> SMIEDVSLPSQVLQDQRLKELNQQLQDQLAQQTPYQNTKPLQDFKHLVVEESPCVTVKEISLIPLIGQSESDLQQFNFVIKAIKKHPQNILGKCIGTQSLHNIVNYAQNELLKKGFITSQIVVSPQDLNHGNLNLSIQIGRLNKIVIQEGKISSLQLKTGLPFKAGDIVNLKRLDQGLENLKRVYAVDMQITPATAQDKELTGYSDLILKLQALQKVNFNLSVDDSGNQDTGTYMGNIGIGINNPFHLNDILSLNVSHSLDDFHESLNRSYFISYQLPVGYYDLGFSYNDYQYRQGTVAPESGYPVIYHGNSQQANLNLSRVISRSGQHKTSVYGKLYHKESQSFLNDIEINVLHRKTSGWNLGVQHRQYLGNAVLDGSIDYRRGMGVGARTAPEENITDVYGNHLPVEGYSRAPLWSADLRYTTPFLLLDKPAQYRLNWRGQYAPKILVPNDRFYIGGRYSVRGFDGELMLSGDNGQYVQQEISLNAPIPNTQFYMAVDQGWVNGRNSIPGQRYLLGSVLGLRTYQNSFYLDAFTGRGLIAPDSIKKDWVTGFSINLSY

CdiB is an outer membrane transporter that releases its CdiA toxin to the cell surface. CdiB proteins are members of the Omp85 superfamily. Despite low sequence similarity (21% sequence identity), both structures adopt a common fold: an N-terminal α-helix (H1) is inserted into the lumen of the β-barrel and is connected by a ~ 20 residue linker to two periplasmic POTRA domains.

We determined two full-length crystal structures of CdiB transporters from Acinetobacter baumannii (strain ACICU) and E. coli (strain EC93), which will be referred to as CdiBAb and CdiBEc. CdiBAb and CdiBEc structures were built and refined to final resolutions of 2.4 Å and 2.6 Å, respectively. However, H1 is positioned very differently in CdiBAb and CdiBEc: the angle between H1 and the β-barrel is about 10° for CdiBAb, versus 25° for CdiBEc. In addition, H1 sits higher in the barrel pore in CdiBAb, positioning its N-terminus closer to the extracellular surface. In this orientation, H1 interacts with the inner barrel wall using 12 H-bonds and three salt bridges, with no interactions to loop 6, for a total buried surface area of 1263 Å2 (Figure 2—source data 1). In CdiBAb, the DxxG motif accounts for four residues on the 12-residue β1 strand, allowing β1 to form an extended β-sheet with β2, β3, and β16. As a result, the β-barrel is in a fully zipped conformation, stabilized by 10 H-bonds between strands β1 and β16. Extracellular loops 1–2 are short, with loop 2 curved inward and partially blocking the top of the channel. As a comparison, when loop 2 adopts an inward conformation in the CdiBAb X-ray structure, the sidechains point in the direction of H1 and loop 6, and the β-barrel lumen is partially capped. The equilibrium simulations demonstrate that CdiBAb interconverts between the two conformations, while CdiBEc stabilizes only the unfolded conformation.GDAP1, a 358-amino-acid mitochondrial outer membrane (MOM) protein regulating the mitochondrial network, is highly expressed in neurons and less in Schwann cells. GDAP1 contains two domains similar to the N- and C-terminal domains of glutathione (GSH) S-transferases (GST) (GST-N and GST-C, respectively), a hydrophobic domain (HD), and a transmembrane domain (TMD). GDAP1 functions in regulating the mitochondrial network by inducing fragmentation of mitochondria without inducing apoptosis. Although the sequence identity is only ∼20%, the GDAP1 core domain shares a fold similar to canonical GST enzymes.

As no GST activity was detected for GDAP1, a metabolite library was screened for GDAP1 binding partners. Through metabolite screening, we identified a ligand for GDAP1, the fatty acid hexadecanedioic acid, which is relevant for mitochondrial membrane permeability and Ca2+ homeostasis. Among ∼300 compounds in a metabolite library, HA showed an effect on GDAP1 stability, increasing its Tm by ∼3 °C. Due to its limited solubility, HA was titrated up to 250 μM, and a concentration-dependent Tm shift was observed. Taken together, DSF, ITC, and BLI all show that HA binds to the GDAP1 core domain and stabilizes its structure. Interestingly, HA binds to GDAP1 in a pocket next to this cluster and forms a hydrogen bond with Arg282. HA binding increases GDAP1 stability by inducing a conformational change of the loop α6-α7, which is involved in the mutation cluster. The HA binding site in the crystal structure of GDAP1 is located close to the CMT-linked residue cluster and the membrane-binding surface. The fatty acid-binding site observed in the GDAP1 crystal structure faces the membrane-binding surface in the context of the modeled full-length dimer, suggesting that the observed ligand could mimic the lipid membrane surface. This, in turn, suggests that membrane binding could affect the conformation of the GDAP1 core domain, for example, via the incorporation of acidic lipid headgroups in the binding site. GDAP1 could be a fatty acid transport protein due to its localization on MAM and MOM and its fatty acid binding shown here.

>[2x]EVKLILYHWTHSFSSQKVRLVIAEKALKCEEHDVSLPLSEHNEPWFMRLNSTGEVPVLIHGENIICEATQIIDYLEQTFLDERTPRLMPDKESMYYPRVQHYRELLDSLPMDAYTHGCILHPELTVDSMIPAYATTRIRSQIGNTESELKKLAEENPDLQEAYIAKQKRLKSKLLDHDNVKYLKKILDELEKVLDQVETELQRRNEETPEEGQQPWLCGESFTLADVSLAVTLHRLKFLGFARRNWGNGKRPNLETYYERVLKRKTFNKVLGHVNNILIS> MNYATVNDLCARYTRTRLDILTRPKTADGQPDDAVAEQALADASAFIDGYLAARFVLPLTVVPSLLKR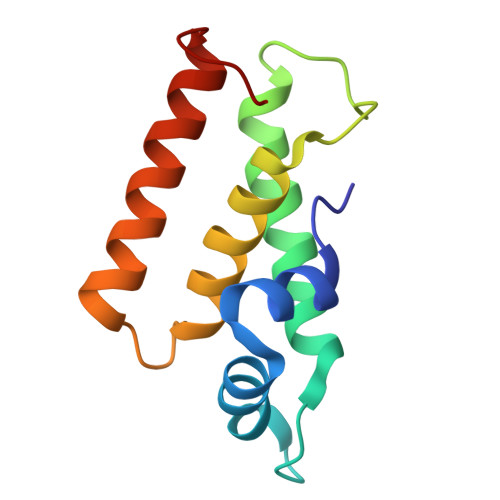QCCVVAWFYLNESQPTEQITATYRDTVRWLEQVRDGKTDPG> ATLKDITRRLKSIKNIQKITKSMKMVAAAKYARAERELKPARVYGVGSLALYEKADIKTPEDKKKHLIIGVSSDRGLCGAIHSSVAKQMKSEAANLAAAGKEVKIIGVGDKIRSILHRTHSDQFLVTFKEVGRRPPTFGDASVIALELLNSGYEFDEGSIIFNRFRSVISYKTEEKPIFSLDTISSAESMSIYDDIDADVLRNYQEYSLANIIYYSLKESTTSEQSARMTAMDNASKNASEMIDKLTLTFNRTRQAVITKELIEIISGAAALD;> AEAAAAQAPAAGPGQMSFTFASPTQVFFNSANVRQVDVPTQTGAFGILAAHVPTLQVLRPGLVVVHAEDGTTSKYFVSSGSVTVNADSSVQLLAEEAVTLDMLDLGAAKANLEKAQSELLGAADEATRAEIQIRIEANEALVKALE;> VAYWRQAGLSYIRYSQICAKAVRDALKTEFKANAMKTSGSTIKIVKVKKE;>DIDTAAKFIGAGAATVGVAGSGAGIGTVFGSLIIGYARNPSLKQQLFSYAILGFALSEAMGLFCLMVAFLILFAM[8x]

Adenosine triphosphate (ATP), the fuel of life, is produced in inner membranes of the mitochondria of eukaryotic cells by an embedded molecular machine with a rotary action, called ATP synthase. Mitochondrial ATP synthases occupy the inner membranes of the organelle and form dimers via specific interactions in their membrane domains. Each monomeric unit in the dimeric bovine enzyme described here is an assembly of 28 polypeptide chains of 17 different kinds, organized into a spherical catalytic globular domain that extends from the inner mitochondrial membrane (IMM) into the mitochondrial matrix, attached to an intrinsic membrane domain by a central stalk and a peripheral stalk (PS). This membrane-bound enzyme is a machine that transmits by a rotary action the potential energy of the transmembrane proton motive force, generated by respiration, into the catalytic sites in the extrinsic domain.

The membrane-bound rotor consists of a ring of eight identical c-subunits in close association with a single static a (or ATP-6) subunit, attached to the asymmetrical central stalk (subunits γ, δ, and ε) which extends from the membrane domain and penetrates into the extrinsic globular catalytic domain along its central axis. Focused local refinement of the rotor (c8-ring plus subunits γ, δ, and ε), the stator (subunits OSCP, b, d, and F6 and associated supernumerary subunits e, f, and g) and the membrane domain (subunits a, A6L, b, d, e, f, g, j, k, and the c8-ring) improved the quality of the maps and the resolutions in these regions to 3.5 to 3.7, 4.2 to 6.0, and 3.6 Å. As it rotates, the asymmetrical central stalk brings about structural changes in the three catalytic sites, found mainly in each of the three β-subunits, which alternate with three noncatalytic α-subunits in the spherical extrinsic domain. The inhibition of ATP hydrolysis in the isolated catalytic F1-domain arrests the rotary cycle at the catalytic dwell, and in structures of the inhibited bovine F1-IF1 complex, the rotary cycle has been arrested at 27° to 32° after the pause in the rotary cycle preceding the release of phosphate. In the current structure, the postphosphate release angles are 28.8°, 26.2°, and 25.5° in states 1 to 3, respectively. Therefore, the rotational angle in the F1-domain is not influenced significantly by interactions with the additional components of the intact enzyme that are absent from the isolated F1-domain. The central cavity of the c8-ring contains a poorly defined, noisy density observed also in the porcine and yeast c-rings (S13 A–E). Here, the upper half of this density has been attributed to a mobile lipid (including possibly coenzyme Q10), and the lower half has been ascribed to another mobile lipid and the C-terminal region of the e-subunit, which extends toward the central cavity on the inter-membrane space (IMS) side of the membrane and could just penetrate into the cavity.>MRGSHHHHHHGSMVVKVGVIGTGAMGRAHIDRLTNVLTGAEVVAVTDIDHEAAEAAVRDFHLNAKVYPDDTSLLQDPDIDAVFVVSFGGAHEATVLKALDTDKFIFTEKPLATTLEGAKRIVDKELTKSKKVIQVGFMRRYDQGIRALKEKLDTGIIGAPLVVRASHINPNVASNYSNEMAITDTLIHEIDEMHWLLDDEYTSIQITYPRQSAEVRNEGLHDPQLATLTTKKGTVIQVLVHVTAQYGYEVKLEVIGETGELQLPNYGLGPILRSNANQQTAVEMSWINRF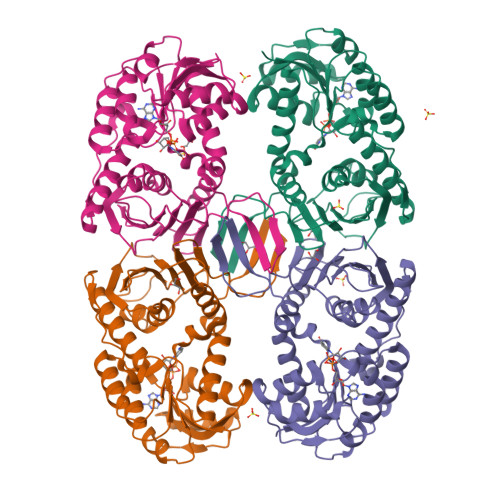IQAYNTEVQEFIDEVAKSEPPVGPSAWDGYIAAITAAAANRSQKDQETVLINVAGTPTFYQ[4x]(1R,2S)-2-{[(pyrrolidin-1-yl)sulfonyl]amino}cyclooctane-1-carboxylic acid | C13 H24 N2 O4 S | 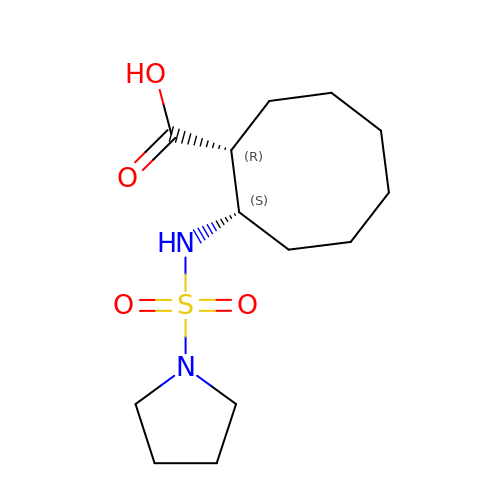SEHSQFUMMWGJHC-NEPJUHHUSA-N>MTIPTLYMNDGMNAQSSQALHIQTYCNSVRQQIPVDFGRFPNLRESERQINTGLGAARQHAEHYLKDIQPLIIRNVTNIQDYFETQNLISTVMPSGATKEQWLSALGMVSDKAKEYQEVSANTRRTIGSLNDKLIIDSNNYQLIVVNLNNVVNGNNGVLEQLNRDIDGINAAIDGAIAGIVVGGLLVIGGAIVTAIGAVAGLVTAGTSTPVVMGGIAMMTAGAGGVIGGAIVLDKSLSAREKLYRDRSQLNSEVLVASQIGSGYRGLQTQAQSAVTAATQMNNAWDSLTSELETLNANLRKGIIDDSFLRQLFLTASQTSVTKVLDGTKIIKQQMA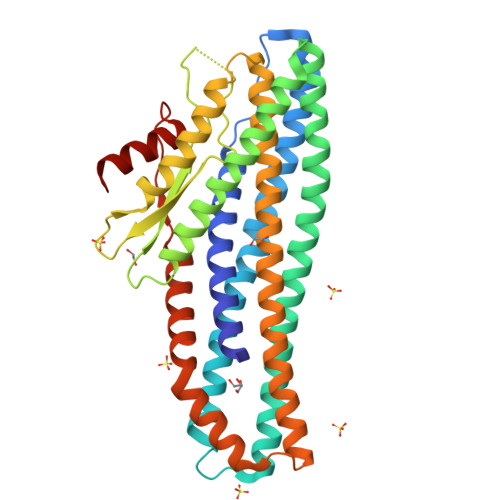GVVVREVPANQSIADFVKRLAALEHHHHHH[2x]> ANSTAELEELLMQRSLTDPQLQAAAAAAADFRILPDATVIKIGGQSVIDRGRAAVYPLVDEIVAARKNHKLLIGTGAGTRARHLYSIAAGLGLPAGVLAQLGSSVADQ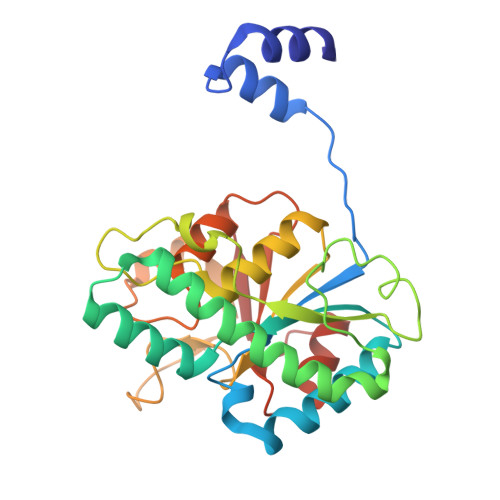NAAMLGQLLAKHGIPVVGGAGLSAVPLSLAEVNAVVFSGMPPYKLWMRPAAEGVIPPYRTDAGCFLLAEQFGCKQMIFVKDEDGLYTANPKTSKDATFIPRISVDEMKAKGLHDSILEFPVLDLLQSAQHVREVQVVNGLVPGNLTRALAGEHVGTIITAS>SRAPAPATPHAPDHSPAPNSPTLTRPPEGPKFPRVKNWELGSITYDTLCAQSQQDGPCTPRRCLGSLVLPRKLQTRPSPGPPPAEQLLSQARDFINQYYSSIKRSGSQAHEERLQEVEAEVASTGTYHLRESELVFGAKQAWRNAPRCVGRIQWGKLQVFDARDCSSAQEMFTYICNHIKYATNRGNLRSAITVFPQRAPGRGDFRIWNSQLVRYAGYRQQDG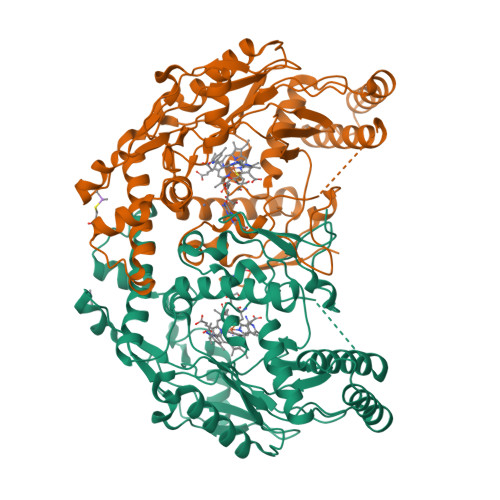SVRGDPANVEITELCIQHGWTPGNGRFDVLPLLLQAPDEAPELFVLPPELVLEVPLEHPTLEWFAALGLRWYALPAVSNMLLEIGGLEFSAAPFSGWYMSTEIGTRNLCDPHRYNILEDVAVCMDLDTRTTSSLWKDKAAVEINLAVLHSFQLAKVTIVDHHAATVSFMKHLDNEQKARGGCPADWAWIVPPISGSLTPVFHQEMVNYILSPAFRYQPDPW[2x]> GVSEIRHTADRWRVSLDVNHFAPDELTVKTKDGVVEITGKHEERQDEHGYISRCF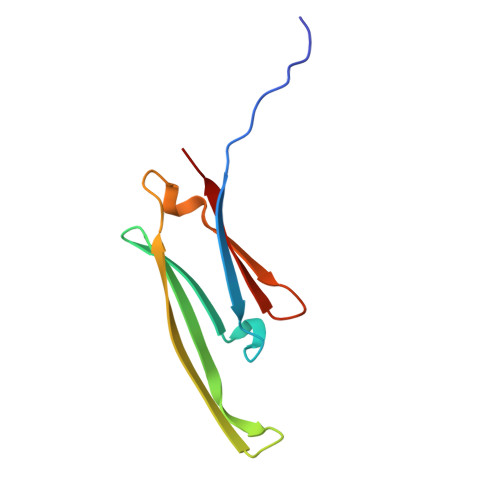TRKYTLPPGVDPTQVSSSLSPEGTLTVEAPMP>[18x]MTTTITIPNSYPIFTPNQVLTNKDLNRVVTYLDEQNRLTRVYLIGMGIVAGMEVSSIYQPGDVNIVVAPGCGITSEGYIISLAETKLTHYQSGVSVPSALFAPSEEQTAASTDQLVELFEQEGNNRLALKNLPDENAFARFLADQTLVVVYELQDQQRDSCLLDCDDTGKDRNFRLRYFLLPRSVPEKLSAEALLQQGFSREPLPQQWRDFSINDIFQAQSSFFQNFFPQVRRFGYTLETPPVIRLSNIVDYDAFLKGYQQVCLQAIDEIDRTFPNLFRLFSPFFSSFNPAPSDFTGLKTLLNQRLSDIVSGSSAENRRSPISQIEAQYALQYFYDYLSQLVSAFRELAESAFDLMDDATPDTRRFPKFLMLGLVPLPNQKPEVYALNSPYRSNFSQSPIYNGNQLRVKQVRFLYDRLVRLCAADSFYLLPFYDTPLKITPSKDRAATLSQQAIPYYLNYPQLYQYWSYDTYRKGRSQSHPAYFYPNNANITPNSDLLHRLDDYSFYRIEGHIGEANATALQRILDYQQRYNLAFDVITLKIGNLQSFQDINISGQFDDLNADFGRIKDTFAKLWQRYEESWSRNVFLYTLKRVFFDKTSLAEIKSDQLFNPIVARASVKEAYEFVKESGDSYRLYLRNAAGIRIARFETVINFSGLSGDSLTQEQERIIGDLLACLPLGKITYGVEPESANNPLSYYLRFSLADELDLPANRGTADISFISLNFFTVNFEGNSPIINQPEFQDFETLYSLLRDVPESSIRVNRLELRMGDRLAADTLNYFELKGLMTAYQQRLAQIMELQLFHKFAQNNPGMEHLGGVPKGGTFVLVYVDGRELVRNLLSADRDPTYQARTEVIKKYASLPPGSPQELATSRELLNREDIVVGDFCLPYRFSSKTPTVSYVLTQPRPIVLLDRTTFCAGDETRYEFILDPTGGTLKGEGSFFADGKYYFQPSRITDDITSETAITFTYVVESSYDTLSVTVYPLPDASFQIKTNFCSNENPVTLRATQPGGNFRAFDSETDISASVINNQEFNPSAVNLGGATEKVITLVYTITSDQGCTNELSRDITIFAVPNATFQVGQGKTRFCSNDEPVDLIARVPGGTFQVRDGAEDISADVINRLTTPPQFDPSAVNLGVAREKVITLEYSISNQGCSNKFTQELRIFAVPNANFRLSTGNRDTFTNNDPPVGLIATQLGGTFQAFDGEEDITADVISPTTPPQFNPSAVNLGDEEEKVITLRYTISNQGCSNNTERRVTIVPPPEVPVRDVEDTSNPDSGDAPTENPIPHPEVRAVNLLAISNNEVINSTNLDGDRTFNLSDFNPNNQYTFEAMTVPEKVNSVIFTYTKPNGSRQALTANTAPYRMPDDWQPSIGIHEIQAQAIREVNGDRLEGATIKVIIRVIDADTDTSPSRSTNPDNLFTRIQNLFPLNRGEIITKIKLPQLLAMSTAIFMLIVGWTYSSSKQVGSTPPSVIKPR;>[6x]MPEYLSISKQKPDFPPYLNFQTLRDIGITHLQALSGKIWTDYNLHDPGVTILEVLCYAITDLGYRNNLDIADLLALNPQDGNSRENNFFTPDAVLTCNPVTELDVRKRLIDIPGVRNAWLQKVTSYEPNIYVNFSDKRLQYNPPTAESKTLNPRGLYTVRLDLDQDYRKNACGQIDRSWGDTLDEVKQVLCDSRNLCEDFADIVILGEEEIGICADIQLETNADAEDVLVNIYVRIQQFLSPRLKFYTLQELLDKGKSPAEIFAGRPSVFDGENRLYKSHGFIDTDELEALTLPTILHTSDLYQEILQVPGVSAIKKLSIANYINGLRQTQGHPWYLQLTDQYRPVLGVKTSKINFFKSELPIGVDEEEVERRYYEQQAAYIKTIRDRDELDIPVPKGSYYDLADHYSIHHDFPTTYGISEDGLPPTVPALRKAQALQLKAYLVFFDQLLASYLAQLSHIRDLFSWEVDVTQPQQNDYATRLQEKQRTYFTQKLDFPEIEKIIPDNYLDVLDEAPETYRDRRNRFLDHLLARFSESFSDYVLLNYQMFATRNNKATQETEIIHDKAQFLQDYPTLSRDRFRAYNYYDCHAVWDTDNVAGFKKRVLRLLGIDDVRRRHLSHYRVDKDSRNLFLSIDFSSDDLTLTSKQRYATTEQAQADQDKLLLFALHPNFYKRLSYKYYYHYSWEILDTQNQSIVRSDRFFPSTKERAAALEPLLQSLLTQLSQLDDTALQNLVITQPTDEDLYSFRLQIPLNSGVITFTGVQRYFSRTEAVDAGVISLRLIQDVQNYRNITLGQDQGTTPQKFTYYGYGLVDHQGSLLSEYTHHFPTELERELSLQRWLTHIQANQNQYKFAIETITNGYVFVINDITNSQTLLRGISSYATEYLAWQAASEFAENLRYLNRYLSPAKDHTGQTYSLGITDKTGKLLAVTTTESDRLLTFQRLNALEPFLVIEAATTPTSGYRYRLVDRQETTILQSIQIYGDETTARDRFYQDVLGTLFETGVINPTTTNKEFGFRILSRPRDTNSVAAIHTQTYTSEAERDAAIEHLLLLVRTARLRISTNSLDSLAYISQIYNPDNQLILQGTQRYTSEDIAWEQGNTLMELAQDEENFRLIDSDDGVYGWELTNEGKDEIFAAQYYNSREERTAAIAEIQKYSNDEGFHLLEHILLRPRTKLPDLTAGDGFLPILVTPEDVNTEPDDPYLLARTDPYSFWVTIVLPYWPQRFRDIPFRRFVERTLRLEAPAHIALKIAWVNVRQMRDFELAYRHWLEQLALESCENAACDLTGTLNRLLKILPQLRNVYPKATLHDCEESSADNNPAILNQTALGTAND;>[18x]MNLRKRNELKSLFKNKSRLSETYFVELIDSTLNKRDDRFHGIWKPGQTYQKGDVVYYNHSLWEMQSENEICAKEEQTPGISTDWKSLLKELEQKVDKLQHELETLHQEFTEYQKQMEIRLQLLARFIPILFIGLGIMFFWLLGQSTVHILAGTT;>[6x]MSNNRDLPKNPLIRDGVSQRQRQVSALSPASIGVDERDLADFLVLVYRLSAKVMYYRAENQPWSPSDADGNWQNFFEGNTPIQIALISKVSPQVVKDIYSQKLAAFLAERTVTSLSEVLSIWKTEILTKIQQWYLGIEAYTPLKSVIKGLVKTNLTEPLMRMQSFELGCGNVDEEFYRGFSGVFGLTIDAPLRSDRTPLMGTVKDARTELDTVFQVLLQTYRQIIQQAPNYLKASLSDRQDHQPFLSLYFAFLEVLQPARDDLNRLTQRHLDFFYRQVLLLPDRPAQADQVHLLFELAKSQREYKLTAGTSFKAGKDATGVDLFYQLDAETVIHKAQIASLKGLFLDSQERKTAAVPQNLTGLYASPVANSVDGKGGAFPQEQIVKTWLPFGNEQRDHARLGVAIASDVLLLQEGRRVVEFKLSLGGFFPRLPDNQLHQAFVVYLSGEKAWIPAPILPVGQLATNGQEQTRWDGSNLYLVVELAADVAPILPYRPDAPIPYDPKELNLPLQLERPIPVARLELNHQLLVNERSPYHYFRDAQILDITVQTRVDEVRNLVVQNDVSVLNPARPFEPFGFQPQDKANLYIGSQEVLQKRLIALTISLELATPKPNNWIEFYAGYDIPANFQPGKVKIQGLRQKTWYPTTANVTANLLDTPEISLTSKLANLKLDSFDQSAPVEMFTPQTKTGFLRLQLSGNFLHEQYPRVLAKQVLAAATNQTVVVSSNQKRQAVIGAYYRRPDKSIFAATTYYVNLDDEPIIPNEPYLPVVRSLSLKYTAQAGMSDCILFHLHPFGGFAKVNLAVNPPLLPYFNQEGELFIGLQNLDPPTALPLLFQVAEETADISLRRQEEYKLQWYYLKDNAWESLGDRIVNDASNGLVTSGIINLGIPADISRNQTTILDPNFHWLKVTIPARSRTVCEIIGVHTQAARVTFKDAGNDPNHLGSPLAGGTISKLAVPQPEVKKIAQPYTSFGGRVKEQPENFYIRISERLRHKGRAVAIFDYERLVLEKFPQIYKVRCINHGQFDDAQEQLYELAPGSVTLAVIPDLSQRSTTNDLEPKVNINLLQEIEKYLASVSSPWAMIKVVNPQYERIQVDFQVKLKAPYSSNFGYYRRELQQAIVGFLTPWTVDSGADINFGGKVYRSSILKFVEEQYYVDYVVNFKMNLNNQQDIREAIAITPRSVITSVSPKTSNQDHMIEEFIEQAIVFNNQKLESGVLGYESLNDLELGE;>[6x]MDDESNAYLGTGWGFPPTFEKKARSVRLVSAEDDIRESLQILLSTNLGERVMQPNYGCNLQDLLFESLSPTVASNIKELVRTAILYYEPRIRLNKLDIQQGISDRQNPSAVNEADAQGLIQIIVDCTIISTNSRFNFVYPFYLQEGSGN;>[3x]MNDRIIPRNSLYDVATFKLLSDGKDITNDYTVLSITVNQIVNRVPTARIILRDGAAADETFAASEGADLVPGQEVEIAAGYDGSDQKIFQGLIVKHALKVTANGDSMLMLDCRGLATKLTVGRHNRYFVDTKDSDAIAEIIAQHSLSADVAATQVQHPEIVQYYATDWDFILSRAEMNGQIVVAQDEKIKVKAPNTSGAPQITLTYGVNLLELEAAMDARHQYQAVKATSWNYADQALVEAEASEPTVNNQGNLSGRQLAQVIDLSALELRHSGLVAEPELKAWADAQLLKSRLAKIQGRVKTKGYPDAKVDVLIQLAGVGDRFNGLAYVSGIRHEIVGGAWDTHIQMGLPPQWFYQEVDIIDKPAAGLLPGVNGLQIGVVVQLQDDPNGEDRILVKVPIIDAQAEGIWARIATLDAGNNRGSFFRPEVGDEVILGFLNDDPRDPVVLGMLNSSAKPAPLRATAENHRKGFFTRSQMQLTFDDDKKIITLQTPGGNKVTISDEDKGITLTDQNGNTFAMSDRGIAMNSPKDITLEATGKLTLKATQDVSIEGLNVNIAANAQFKAQGNAGAEVSSSAIAVLKGSLVMIN;>[6x]MALTKVKLLAYQDKRFENKLGEFELPINPEQFSQSFKVEYNREQAQGSQRNDPEFKFTKPEELKLDFTFDGTGVVPVNNGKPGEFHQDVADQVRVFLDLVYSMNSETHKPNFLRLIWGDFSFGEKNGFDCLLTDLQINYTLFDQTGKPLRAKLSTTFTSYVEQNRRVREEGKQSPDVTHQRKVKAGDTLPLMTHRIYGDPAYYLQIAKVNGLINFRKLATNTDLRFPPLEKTQS;>[3x]MPLEIRELVIKASVNEGGQNQGTGGAGDQSAIIAACVEQVLAILQEKSER;>MIRTYPPVSFFFEVVFQGENLDKDVVETRFQSVTGLSVDMQTETLKEGGENRFEHILPVRTKYDPLVLKRGLVNDSQMVKWCMDAILNFDIRPMNLLVRLLHIERSDPNQPPEAIATGGSSTIAPLMTWKVINAWPKKWSVSEFNAEQNSIAVESLELNYSYFETLK[6x];>MAEYPLPKFHFQVDWGGSRLGFTEVSGLDVETEVIEYREGNLPQYHKLKMPGMQKFSNITMKRGTFQGDNDFYKWWNTVALNTIERRDLTISLLNEKHEPVVVWKVNRAWPTKVQSTDLKGDGNEVAIESIEVAHEGLTIQNG[6x];>MPSTYKTPGVYIEEISKFPPSIAQVETAIPAFIGYTQIAKVGVENFHTDADNLILRPVRITSLLEYEQFFGKAINETTIQVVIQDTTDSRGNLTERKASARITSPSPHNLYYSMQAYFANGGGPCYIVSVGPMSNTGTIQLEALQNGLAEVAKEDEVTLLVFPESQSLSDENYAALMSAALEQCANLQDRFTVMDLKLPATRPIPANAIVGASNAFRDLSLPQDNLKYGACYAPDIETIFNYFYQEDAVTIFRSVNGGAEEQDTLTMAGYNPANGGDGIQYALIESAIDQLPLILPPSPLVVGQYARTDNTRGVWKAPANVALSSVIKPVLKITNEQQNNLNVHPTGKSINAIRAFTGKGTLIWGARTLAGNDNEWRYVSVRRFFNMAEESIKKGSEPFVFEPNDANTWTKVKAMIENFLTLQWRAGALAGAKPEQAFYVKIGLNETMTALDILEGRMIVEIGMAVVRPAEFIILKFSHKMQES[18x]

Contractile injection systems (CISs) are a diverse, yet evolutionarily related, group of assemblies that mediate bacterial cell–cell interactions. Their contractile apparatus is homologous to contractile phage tails, using a contractile outer sheath to propel an effector-loaded tube into target cells. Here, we characterized a CIS in the multicellular cyanobacterium Anabaena, with features distinct from extracellular CISs and T6SSs. In contrast to cytoplasmic free-floating eCISs and cytoplasmic membrane-anchored T6SSs, Anabaena CISs are anchored to the TM, which is mediated by modified tail fibres and a baseplate component.

The resulting maps of the baseplate and of the distal end cap reached resolutions of ~2.9 and ~2.8 Å, respectively. The transition from the inner tube with C6 symmetry to Cis8, the VgrG-like spike with C3 symmetry, was facilitated by Cis5 and Cis7, which formed the first two layers of the inner tube. The cavity of the spike towards the tube lumen was plugged by three copies of Cis6. The highly conserved baseplate component Cis9 linked the lateral baseplate components Cis11 and Cis12 to the first layer of the sheath. Cis11 and Cis12 formed a hexamer of heterodimers surrounding the spike as seen in previously studied CISs. When compared to Afp11/Pvc11, Cis11 harboured three extra domains including an extended carboxy terminus. The second additional Cis11 domain seemed to stabilize interactions with Cis12, whereas the third extra domain composed the cage surrounding the spike, which was observed in the in situ structure. The cage was further surrounded by the crown, consisting of six trimers of Cis19, which are not present in other studied CISs. The wide connector observed in the in situ subtomogram average was composed of an extra domain of the baseplate component Cis12. The amino-terminal domains of Cis13 proteins bound the baseplate while the C termini formed a triple alpha helix extending towards the TM and penetrating it.>[2x]MADLQHIKHMRTAVRLARYALDHDETPVACIFVHTPTGQVMAYGMNDTNKSLTGVAHAEFMGIDQIKAMLGSRGVVDVFKDITLYVTVEPCIMCASALKQLDIGKVVFGCGNERFGGNGTVLSVNHDTCTLVPKNNSAAGYESIPGILRKEAIMLLRYFYVRQNERAPKPRSKSDRVLDKNTFPPMEWSKYLNEEAFIETFGDDYRTCFANKVDLSSNSVDWDLIDSHQDNIIQELEEQCKMFKFNVHKKSKV;>GPHMASMVKKVNNPLKIDYQNGIIENRLLQIRNFKDVNTPKLINVWSIRIDPRDSKKVIELIRNDFQKNDPVSLRHLKRIRKDIETSTLEVVLCSKEYICDEGEINNKLKSIWVGTKKYELSDDIEVPEFAPSTKELNNAWSVKYWPLIWNGNPNDQILNDYKIDMQEVRNELSRASTLSVKMATAGKQFPMVSVFVDPSRKKDKVVAEDGRNCENSLPIDHSVMVGIRAVGERLREGVDEDANSYLCLDYDVYLTHEPCSMCSMALIHSRVRRVVFLTEMQRTGSLKLTSGDGYCMNDNKQLNSTYEAFQWIGEEYPVGQVDRDVCC[2x]

The adenosine-to-inosine (A-to-I) editing in anticodons of tRNAs is critical for wobble base-pairing during translation. This modification is produced via deamination on A34 and catalyzed by the adenosine deaminase acting on tRNA (ADAT) enzyme. By contrast, in eukaryotic organisms like yeasts, ADAT is a heterodimer formed by ADAT2 and ADAT3 (the ScADAT2/3 heterodimer). ADAT2 is the catalytic subunit, and ADAT3 serves only a structural role, because the essential glutamate in the conserved H(C) XE motif of the latter is usually mutated to a catalytically inactive residue (a valine in the ScADAT3 case).

In this study, we determined a crystal structure of the ScADAT2/3 heterodimer to 2.8 Å and revealed the assembly of the eukaryotic ADAT enzymes. There are two ScADAT2 (chains A and B) and two ScADAT3 copies (chains C and D) in the asymmetric unit, forming two heterodimers. The ScADAT2 and ScADAT3 subunits of the heterodimer make substantial contacts, exclusively through the ScADAT2-CD/ScADAT3-PCD interface, burying a total surface area of 2010 Å2. Like SaTadA, the active site of ScADAT2 comprised a zinc ion coordinated by four ligands: His54, Cys88, Cys91, and a water molecule. Importantly, while the C-terminal half of ScADAT3 forms a pseudo-catalytic domain (PCD), resembling TadA, the eukaryote-specific N-terminal sequence forms a stand-alone domain and functions as a tRNA-binding domain. Full-length ScADAT2/3 showed a strong binding capacity to the tRNAAla substrate, but the tRNA binding affinity for the ScADAT3/ΔAsp30-Pro148 mutant (the ScADAT3 N-lobe deletion mutant with the removal of residues Asp30-Pro148 from ScADAT2/3, designated as Del30-148) was completely lost, underscoring the importance of RLD to tRNA binding. We also discovered the zinc-binding site in ScADAT3, which is coordinated by four ligands: His216, Cys254, Cys257, and Cys322. Cys322, the last residue in the ScADAT3 coding sequence, forms the fourth ligand using its side chain and replaces the catalytic water molecule as found in ScADAT2. Surprisingly, we found that the tRNA entrance into PCD is blocked by ScADAT3 itself. Specifically, the last fragment of ScADAT3 (Trp306-Cys322) forms a loop and winds back into the pseudo-active site.The protein kinase CLK1 (cdc2-like kinase1) modulates activity of SPF45 by regulating its expression and by phosphorylating the protein at distinct serine residues. The CLK protein kinase family is closely related both in structure and function to the family of dual-specificity tyrosine phosphorylation-regulated kinases (DYRKs). The ATP binding pockets of CLK1 and DYRK1A are rather similar both in terms of sequence and surface shape. 3-Aryl-substituted 6,7-dihydropyrrolo[3,4-g]indol-8(1H)-ones were identified as inhibitors of the CLK protein kinase family.

The 2-brominated derivative 16 was prepared by reaction of 8a with N-bromosuccinimide. The structure analysis revealed a binding mode resembling the orientations of 8g in CLK1 and of 8a in CLK3. While the lactam substructure of 16 forms hydrogen bonds to the hinge region, the indole nitrogen is connected to the hinge via hydrogen bonds through a water molecule. The planes of the phenyl substituents in 8g and 16 are nearly perpendicularly oriented in the two structures. In both complexes, three water molecules occupy the area near the Lys191 and Glu206 side chains. For accommodation of the bromo substituent of 16, the entrance to the ATP pocket is somewhat widened compared to the situation found with 8g. Substitution of the parent structure 8a at position 2 by either methyl (8k) or bromine decreased the selectivity towards the DYRK family more than tenfold.

>SMHLICQSGDVLSARYEIVDTLGEGAFGKVVECIDHKAGGRHVAVKIVKNVDRYCEAARSEIQVLEHLNTTDPNSTFRCVQMLEWFEHHGHICIVFELLGLSTYDFIKENGFLPFRLDHIRKMAYQICKSVNFLHSNKLTHTDLKPENILFVQSDYTEAYNPKIKRDERTLINPDIKVVDFGSATYDDEHHSTLVSTRHYRAPEVILALGWSQPCDVWSIGCILIEYYLGFTVFPTHDSKEHLAMMERILGPLPKHMIQKTRKRKYFHHDRLDWDEHSSAGRYVSRACKPLKEFMLSQDVEHERLFDLIQKMLEYDPAKRITLREALKHPFFDLLKKSI[3x]> MKTQVAIIGAGPSGLLLGQLLHKAGIDNVILERTTPDYVLGRIRAGVLEQGMVDLLREAGVDRRMARDGLVHEGVEIAFAGQRRRIDLKRLSGGKTVTVYGQTEVTRDLMEAREASGATTVYQAAEVRLHDLQGERPYVTFERDGERLRLDCDYIAGCDGFHGISRQSIPAERLKVFERVYPFGWLGLLADTPPVSHELIYANHPRGFAL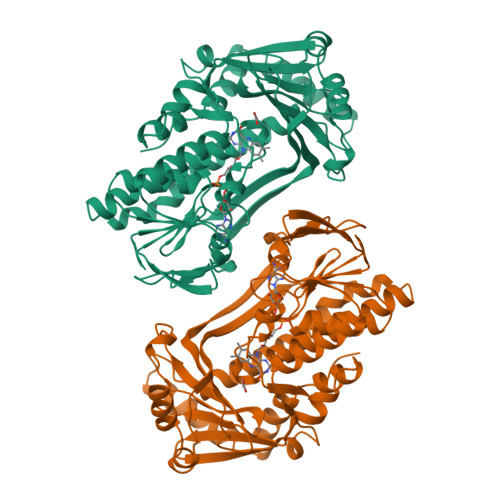CSQRSATRSRYYVQVPLTEKVEDWSDERFWTELKARLPAEVAEKLVTGPSLEKSIAPLRSFVVEPMQHGRLFLAGDAAHIVPPTGAKGLNLAASDVSTLYRLLLKAYREGRGELLERYSAICLRRIWKAERFSWWMTSVLHRFPDTDAFSQRIQQTELEYYLGSEAGLATIAENYVGLPYEE> MRKYAAIALCTSAILAGCNTSNVSQEPKKEKKVQEVAIQKEALQEQGKISYTPITHESTNTSIHI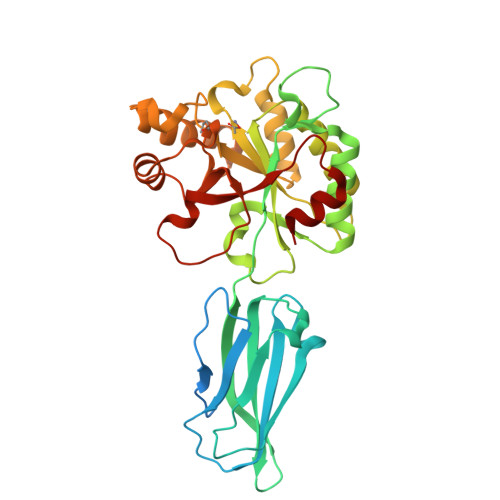TDLKDSLNEVQYKIWRTADGKERAKSFSSKEKEKQFTIPFDIKEFEGKRGEFQIEATGMKEDGKTIPLTKSIITFEQKVPVLMYHAIDDYHGQGIKDLFVSPANFEAQMKHLKDNGYTLLTFERWGDINKVNKPIFVTFDDGMKNNMNAFRVLQKLKDDTFKPAATEYMIVDNVDVEGALSTSEIKEMVDSGIFSVQSHTATHADLPKITNYEEELKGSKEKLEKITGKPVIAIAYXFGHVDDKVVTETKKYYQFATTTKPGQFITKGEPDELLKMKRVRIHHTTTVEQFASSIK>[2x]MTSNNLPTVLESIVEGRRGHLEEIRARIAHVDVDALPKSTRSLFDSLNQGRGGARFIMECKSASPSLGMIREHYQPGEIARVYSRYASGISVLCEPDRFGGDYDHLATVAATSHLPVLCKDFIIDPVQVHAARYFGADAILLMLSVLDDEEYAALAAEAARFDLDILTEVIDEEEVARAIKLGAKIFGVNHRNLHDLSIDLDR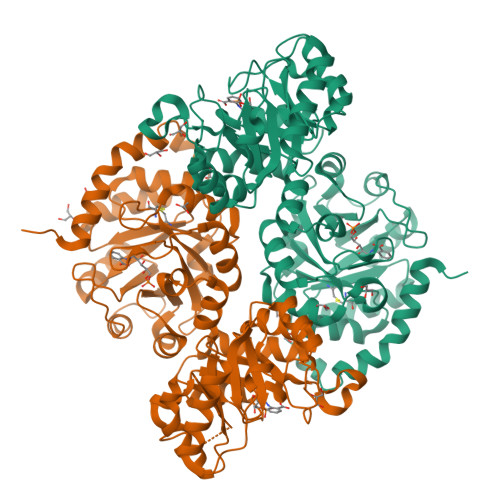SRRLSKLIPADAVLVSESGVRDTETVRQLGGHSNAFLVGSQLTSQENVDLAARELVYGPNKVCGLTSPSAAQTARAAGAVYGGLIFEEASPRNVSRETLQKIIAAEPNLRYVAVSRRTSGYKDLLVDGIFAVQIHAPLQDSVEAEKALIAAVREEVGPQVQVWRAISMSSPLGAEVAAAVEGDVDKLILDAHEGGSGEVFDWATVPAAVKAKSLLAGGISPDNAAQALAVGCAGLDINSGVEYPAGAGTWAGAKDAGALLKIFATISTFHYLEHHHHHH>MLLVKAVKVLVMGGCMLPIAFGALGTGVLFAGFNVALSRNPEETESLFNNTLMGFALIETFIFMSIGLGFFVLFAA[10x];> MFTRFVTQPTLLTQTQRALFSALTKKQKMEVTLRTPYKEYLANFDGFSRITAKTNEASLVIQNKTPASLYVLPPGPLKIRFTSEVKNVSGDFLHTGGWVIVHADNTCEINVMDLFDRKEVRADQFEKGNIQDLDTLAGKYAAKSRKSTVRLFTKATTQ;> MCIEFAFKKAGIPIVRNFLHSTEGVIYGLPQRVQRNLAINYTVKQYKEGKAVSAKTIKTLQEAFPSKGDTK;> MFGLASKGFINTSLVMVPQMNFGANLKQLKIRMKAIGSIKKITKAMKMVAASKMKAETSRLENGRNFAVGSVQKMLENESYVQKKKSTTAPKSTLLVPITSDKGLCGSVNSSIVREVKRLALNNRSAFGLLPVGEKGSSGLSRPFPDLLKSSIVNIQNVNFPTAA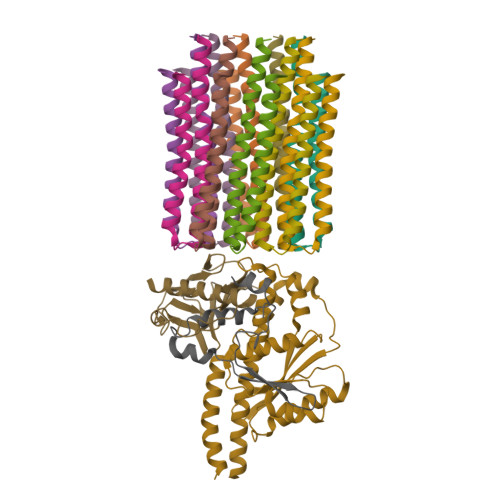AIAHQVSTQGAGYDQVTLIYNHFKNAISYVVKHQELLPRAQFLNLFKYVTRHEAVEPELEYSKNYFFELYMASSVYNALLNSSASEQASRMNAMENASKNAGEILSKLTLDYNKARQAKITMELIEIISGASIV> MDINELIIGAQSADKHTREVAETQLLQWCDSDASQVFKALANVALQHEASLESRQFALLSLRKLITMYWSPGFESYRSTSNVEIDVKDFIREVLLKLCLNDNENTKIKNGASYCIVQISAVDFPDQWPQLLTVIYDAISHQHSLNAMSLLNEIYDDVVSEEMFFEGGIGLATMEIVFKVLNTETSTLIAKIAALKLLKACLLQMSSHNEYDEASRKSFVSQCLATSLQILGQLLTLNFGNVDVISQLKFKSIIYENLVFIKNDFSRKHFSSELQKQFKIMAIQDLENVTHINANVETTESEPLLETVHDCSIYIVEFLTSVCTLQFSVEEMNKIITSLTILCQLSSETREIWTSDFNTFVSKETGLAASYNVRDQANEFFTSLPNPQLSLIFKVVSNDIEHSTCNYSTLESLLYLLQCILLNDDEITGENIDQSLQILIKTLENILVSQEIPELILARAILTIPRVLDKFIDALPDIKPLTSAFLAKSLNLALKSDKELIKSATLIAFTYYCYFAELDSVLGPEVCSETQEKVIRIINQVSSDAEEDTNGALMEVLSQVISYNPKEPHSRKEILQAEFHLVFTISSEDPANVQVVVQSQECLEKLLDNINMDNYKNYIELCLPSFINVLDSNNANNYRYSPLLSLVLEFITVFLKKKPNDGFLPDEINQYLFEPLAKVLAFSTEDETLQLATEAFSYLIFNTDTRAMEPRLMDIMKVLERLLSLEVSDSAAMNVGPLVVAIFTRFSKEIQPLIGRILEAVVVRLIKTQNISTEQNLLSVLCFLTCNDPKQTVDFLSSFQIDNTDALTLVMRKWIEAFEVIRGEKRIKENIVALSNLFFLNDKRLQKVVVN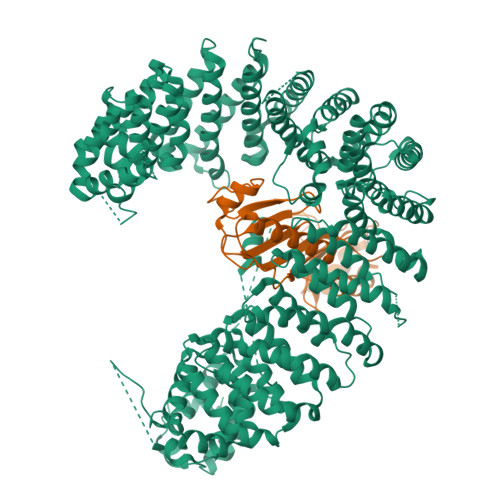GNLIPYEGDLIITRSMAKKMPDRYVQVPLYTKIIKLFVSELSFQSKQPNPEQLITSDIKQEVVNANKDDDNDDWEDVDDVLDYDKLKEYIDDDVDEEADDDSDDITGLMDVKESVVQLLVRFFKEVASKDVSGFHCIYETLSDSERKVLSEALL;> SGIVPTLQNIVATVTLGCRLDLKTVALHARNAEYNPKRFAAVIMRIREPKTTALIFASGKMVVTGAKSEDDSKLASRKYARIIQKIGFAAKFTDFKIQNIVGSCDVKFPIRLEGLAFSHGTFSSYEPELFPGLIYRMVKPKIVLLIFVSGKIVLTGAKQREEIYQAFEAIYPVLSEFRKM>MSKEVSEEAQAHQHGKDYVDPPPAPFFDLGELKLWSFWRAAIAEFIATLLFLYITVATVIGHSKETVVCGSVGLLGIAWAFGGMIFVLVYCTAGISGGHINPAVTFGLFLARKVSLLRALVYMIAQCLGAICGVGLVKAFMKGPYNQFGGGANSV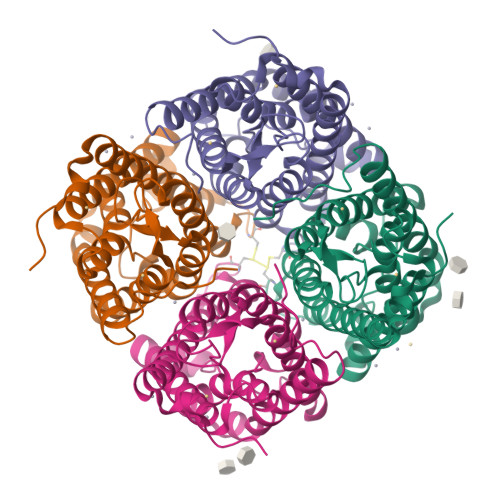ALGYNKGTALGAEIIGTFVLVYTVFSATDPKRSARDSHVPILAPLPIGFAVFMVHLATIPITGTGINPARSFGAAVIFNSNKVWDDQWIFWVGPFIGAAVAAAYHQYVLRAAAIKALGSFRSNPTN[8x]> GSHMASS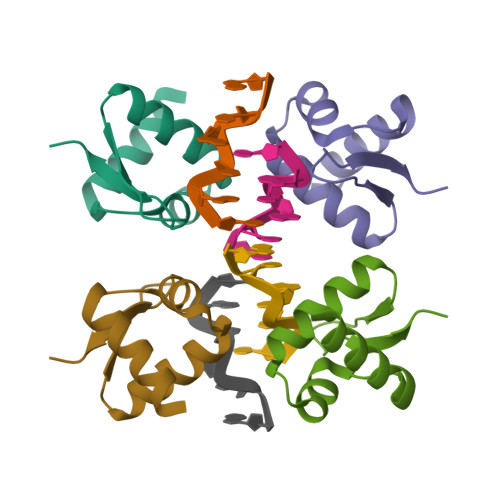AENEIEMRICDYLRRHGRSTVQDIFKELKLEKSTVNRHLYSLQASKQVFKTVEDNKRPVWNLVES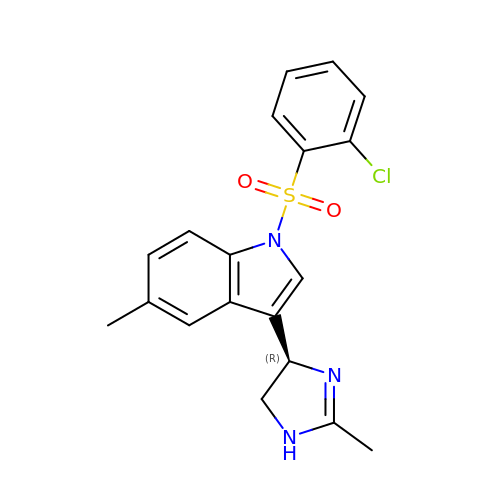1-[(2-chlorophenyl)sulfonyl]-5-methyl-3-[(4R)-2-methyl-4,5-dihydro-1H-imidazol-4-yl]-1H-indole | C19 H18 Cl N3 O2 S | QKLXECCUITXSOU-KRWDZBQOSA-N>[4x]MNTINIAKNDFSDIELAAIPFNTLADHYGERLAREQLALEHESYEMGEARFRKMFERQLKAGEVADNAAAKPLITTLLPKMIARINDWFEEVKAKRGKRPTAFQFLQEIKPEAVAYITIKTTLACLTSADNTTVQAVASAIGRAIEDEARFGRIRDLEAKHFKKNVEEQLNKRVGHVYKKAFMQVVEADMLSKGLLGGEAWSSWHKEDSIHVGVRCIEMLIESTGMVSLHRQNAGVVGQDSETIELAPEYAEAIATRAGALAGISPMFQPCVVPPKPWTGITGGGYWANGRRPLALVRTHSKKALMRYEDVYMPEVYKAINIAQNTAWKINKKVLAVANVITKWKHCPVEDIPAIEREELPMKPEDIDMNPEALTAWKRAAAAVYRKDKARKSRRISLEFMLEQANKFANHKAIWFPYNMDWRGRVYAVSMFNPQGNDMTKGLLTLAKGKPIGKEGYYWLKI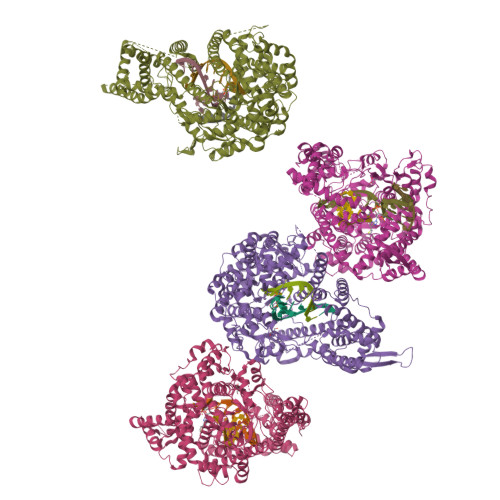HGANCAGVDKVPFPERIKFIEENHENIMACAKSPLENTWWAEQDSPFCFLAFCFEYAGVQHHGLSYNCSLPLAFDGSCSGIQHFSAMLRDEVGGRAVNLLPSETVQDIYGIVAKKVNEILQADAINGTDNEVVTVTDENTGEISEKVKLGTKALAGQWLAYGVTRSVTKRSVMTLAYGSKEFGFRQQVLEDTIQPAIDSGKGLMFTQPNQAAGYMAKLIWESVSVTVVAAVEAMNWLKSAAKLLAAEVKDKKTGEILRKRCAVHWVTPDGFPVWQEYKKPIQTRLNLMFLGQFRLQPTINTNKDSEIDAHKQESGIAPNFVHSQDGSHLRKTVVWAHEKYGIESFALIHDSFGTIPADAANLFKAVRETMVDTYESCDVLADFYDQFADQLHESQLDKMPALPAKGNLNLRDILESDFAFA> SLLNVPAGKDLPEDIYVVIEIPANADPIKYEID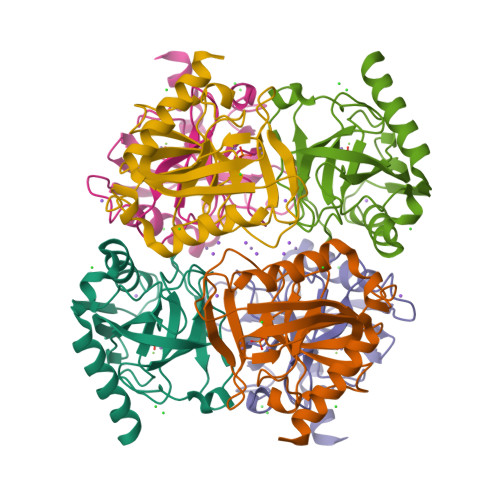KESGALFVDRFMSTAMFYPCNYGYINHTLSLDGDPVDVLVPTPYPLQPGSVTRCRPVGVLKMTDEAGEDAKLVAVPHSKLSKEYDHIKDVNDLPELLKAQIAHFFEHYKDLEKGKWVKVEGWENAEAAKAEIVASFERAKNK> ASMTGGQQMGRDEAGITGTWYNQLGSTFIV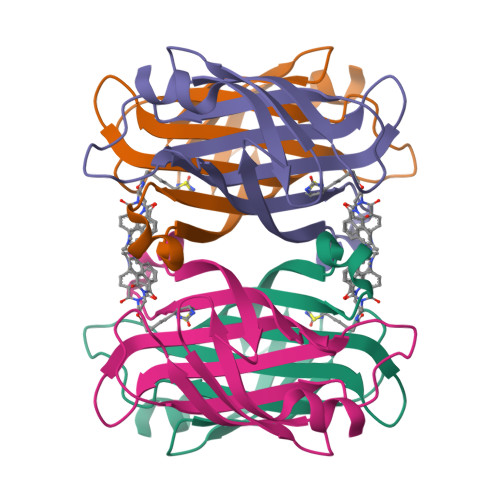TAGADGALTGTYESAVGNAESRYVLTGRYDSAPATDGSGTALGWTVAWKNNYRNAHSATTWSGQYVGGAEARINTQWLLTSGTTEANAWKSTLVGHDTFTKVKPSAASIDAAKKAGVNNGNPLDAVQQ> SPIENEDFCAVCINGGELLCCDRCPKVYHLSCHVPALLSFPGGEWVCTLCRSLTQPEMEYDCENARYGHPGVRV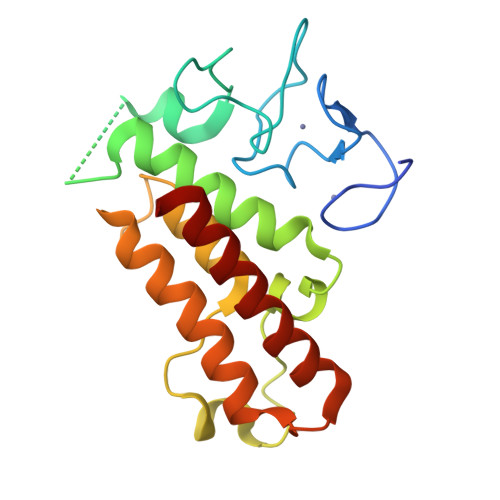LPGLSMYDQKKCEKLVLSLCCNSLSLPFHEPVSPLARHYYQIIKRPMDLSIIRRKLQKKDPAHYTTPEEVVSDVRLMFWNCAKFNYPDSEVAEAGRCLEVFFEGWLKEIYP>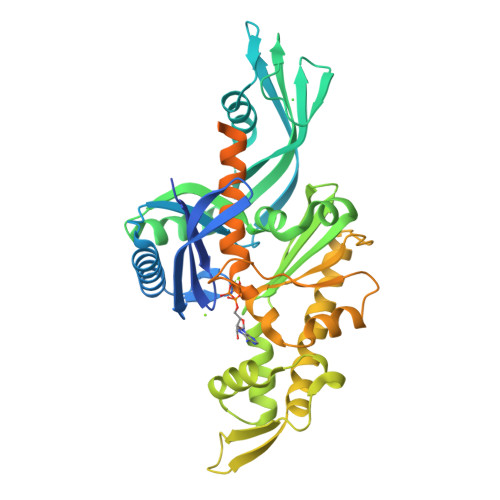[4x]MNHKVHHHHHHIEGRHMEEHYYVSIDIGSSSVKTIVGEKFHNGINVIGTGQTYTSGIKNGLIDDFDIARQAIKDTIKKASIASGVDIKEVFLKLPIIGTEVYDESNEIDFYEDTEINGSHIEKVLEGIREKNDVQETEVINVFPIRFIVDKENEVSDPKELIARHSLKVEAGVIAIQKSILINMIKCVEACGVDVLDVYSDAYNYGSILTATEKELGACVIDIGEDVTQVAFYERGELVDADSIEMAGRDITDDIAQGLNTSYETAEKVKHQYGHAFYDSASDQDIFTVEQVDSDETVQYTQKDLSDFIEARVEEIFFEVFDVLQDLGLTKVNGGFIVTGGSANLLGVKELLSDMVSEKVRIHTPSQMGIRKPEFSSAISTISSSIAFDELLDYVTINYHDNEETEEDVIDVKDKDNESKLGGFDWFKRKTNKKDTHENEVESSDEEIYQSEDNHQEHKQNHEHVQDKDKEESKFKKLMKSLFE> GLRHTFVVADATLPDCPLVYASEGFYAMTGYGPDEVLGHNCRFLQGEGTDPKEVQKIRDAIKKGEACSVRLLNYRKDGTPFWNLLTVTPIKTPDGRVSKFVGVQV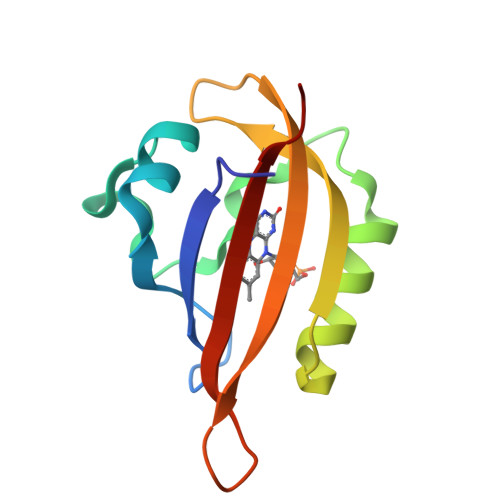DVTS> GPSTEDVPGDPQDVKATPLNSTSIHVSWKPPLEKDRNGIIRGYHIHAQELRDEGKGFLNEPFKFDVVDTLEFNVTGLQPDTKYSIQVAALTRKGDGDRSAAIVVKTPGGVP

An understudied class of proteins in phosphotyrosine signaling, the receptor protein tyrosine phosphatases (RPTPs), are a family of single-pass transmembrane proteins whose architecture include an extracellular domain resembling those of cell adhesion molecules (CAMs) and intracellular single or tandem tyrosine phosphatase domains. In vertebrates, this diversity is typified by the leukocyte common antigen related (Lar) and its two homologs RPTPδ/PTPRD and RPTPσ/PTPRS, which form the type IIa family of RPTPs. The ectodomains of Lar-RPTPs resemble immunoglobulin (Ig)-superfamily CAMs and include three Ig-like domains followed by four to nine fibronectin type III (FN) repeats. Surprisingly, we uncovered a tripeptide, Lys-Gly-Asp (KGD), in the Dlar FN5 domain that is similar to the RGD motif in FN10 and is conserved in the Lar-RPTP homologs across species.

To determine if Dlar possesses the structural characteristics of an integrin ligand, we sought to find a crystallizable region of the Dlar extracellular region encompassing the FN5 domain. Proteins including the FN4-FN6, FN4-FN5, and FN5 were soluble, but only the FN5 yielded diffraction quality crystals. Interestingly, a ~5 molar equivalent of Zn2+ was required to grow diffraction-quality crystals of Dlar FN5. We used the anomalous signal from bound Zn2+ ions to calculate experimental phases and obtain an initial model. The final structure was refined to a resolution of 1.3 Å. Overall, the Dlar FN5 adopts a prototypical β-sandwich fold described for FN domains with two Zn2+ ions. The first Zn2+ is bound by His-745 in strand C and Asp-766 at a crystal contact and may be an artifact of crystallization. The second is coordinated by residues within a single FN5 domain, including the Asp-796 from the KGD motif and two histidine residues, His-745 and His-747. Although the KGD of Dlar lies in the same general area, the side chains are not as accessible for binding with the Asp-796 positioned against the β-strand and the Lys-794 pointing back toward the molecule instead of accessible in the solvent. Importantly, the KGD does not extend away from the domain as seen in FN10.> GLGDELEEVIVEKTKQTVASISSGPKHTQKVPILTANETGATMPVLPSDSIETRTTYMHFNGSETDVECFLGRAACVHVTEIQNKDATGIDNHREA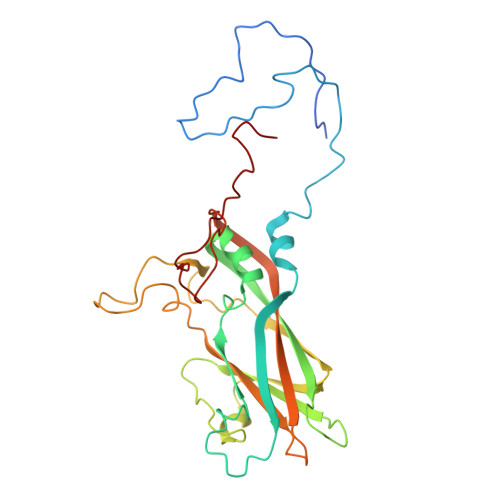KLFNDWKINLSSLVQLRKKLELFTYVRFDSEYTILATASQPDSANYSSNLVVQAMYVPPGAPNPKEWDDYTWQSASNPSVFFKVGDTSRFSVPYVGLASAYNCFYDGYSHDDAETQYGITVLAHMGSMAFRIVNEHDEHKTLVKIRVYHRAKHVEAWIPRAPRALPYTSIGRTNYPKNTEPVIKKRKGDIKSY> AEALSNPGALDLPSLTSLLSEKAKEFLMENRVQSFYQQELEMVESLLSLANQPVIHSASSDQVNFKKDTTSKAIHSIFKNAIQLLQEKGLVFQKDDGFDNLYYVTREDKDLHRKIHRIIQQDCQKPNHMEKGCHFLHILACARLSIRPGLSEAVLQQVLE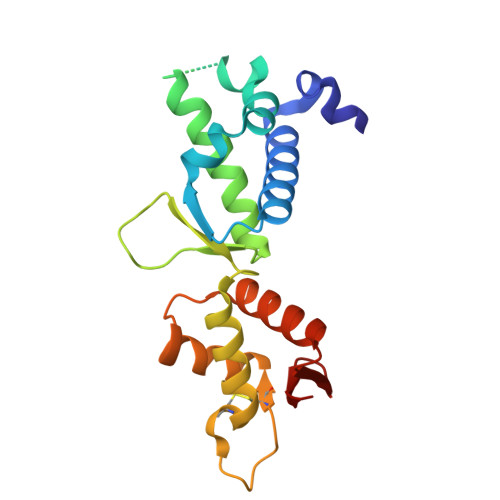LLEDQSDIVSTMEHYYTAF OmpK36 GD, referred to as simply ‘OmpK36’, is a 373 amino acid outer membrane porin from Klebsiella pneumonia involved in nutrient and antibiotic diffusion in gram negative bacteria, while Cld is a heme-b-containing homodimeric oxidoreductase from Cyanothece sp. PCC7425, consisting of 181 amino acids per monomer. The effectiveness of AnACor is demonstrated for long-wavelength data sets collected at 3.54 Å, on a crystal of the membrane protein OmpK36 GD, and at 4.13 Å, on a crystal of the heme-binding enzyme chlorite dismutase (Cld). The choice of these two samples for this study was motivated by their crystallization in low-symmetry space groups, posing a challenge for the conventional absorption correction methods used in standard X-ray diffraction scaling programs.

In addition to three methionines and one cysteine per polypeptide chain, each Cld monomer also binds an Fe-containing heme ligand and a Cl− anion. A single SO4 2− anion could be identified for the dimer, bringing the total number of anomalous scatterers to 13. For Cld, the merging R factors, I/σ(I) and anomalous slopes are noticeably better for AC compared with SH. In contrast to OmpK36, where data quality indicators changed little between the SH and AC strategies, for Cld, the analytical absorption correction strategy (AC) gives substantially better data statistics compared with SH. For instance, in terms of the merging R factors, we observe a decrease of the R merge from 0.163 with SH to 0.112 with AC and a further decrease to 0.095 with the ACSH treatment. The anomalous slope value increases from 1.36 with SH to 2.48 and 2.5 for AC and ACSH, respectively. This indicates an impressive improvement in the anomalous signal as a result of applying analytical absorption corrections. For the largest peaks, MET99 and CYS132, we observe increases in peak heights from 14 to 17 and 18σ for AC and ACSH, respectively. However, while the difference between AC and ACSH is small, they outperform the spherical harmonics correction. This is in particular reflected in the outcome from experimental phasing, where two data sets are sufficient for both AC and ACSH, while three data sets are needed to solve the structure from data corrected by SH.

>[2x]GPGYQDPNNRYSFIGGRTGQWQVVKIRNVLGPGLQLVEKVNILNGAVAEIPLDSAWRLQGFASNIRYAIRTELEALQAVQPMLNRAEAILAVLIPIKKSAQWWEMAQDERRDIFERESHHTAVGLEYLPGVARRLLHCRDLGEEFDFLTWFEFAPEHSSAFNELLLRMRASKEWEYVEREVEVWLKRL>[4x]SNANYMETGDQRFGDLVFRQLAPNVWQHTSYLDMPGFGAVASNGLIVRDGGRVLVVDTAWTDDQTAQILNWIKQEINLPVALAVVTHAHQDKMGGMD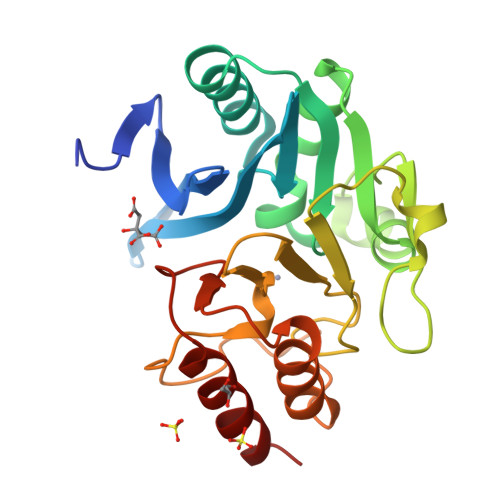ALHAAGIATYANALSNQLAPQEGMVAAQHSLTFAANGWVEPATAPNFGPLKVFYPGPGHTSDNITVGIDGTDIAFGGCLIKDSKAKSLGNLGDADTEHYAASARAFGAAFPKASMIVMSHSAPDSRAAITHTARMADKLR>MALSQATDPFRAAVEFTLMPMLITNPHLPDNPIVFANPAFLKLTGYEADEVMGRNCRFLQGHGTDPAHVRAIKSAIAAEKPIDIDIINYKKSGEAFWNRLHISPVHNANGR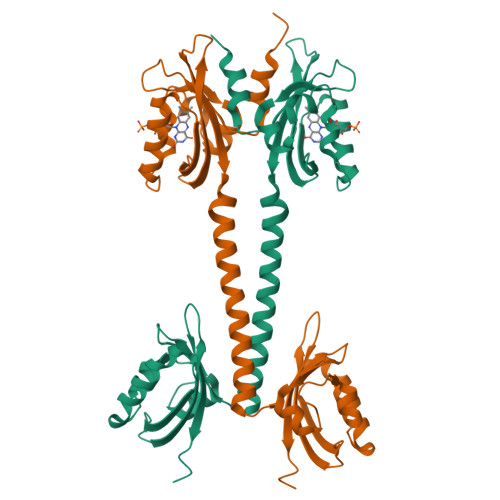LQHFVSSQLDVTLELSRLVELEKERKTLSIETARSKDQLDYIVEVANIGFWTREFYSGKMTCSAECRRIYGFTPDEPVHFDTILDLVVLEDRMTVVQKAHQAVTGEPYSIEYRIVTRLGETRWLETRAKALTGENPLVLGIVQDVTERKHHHHHH[4x]Bdellovibrio bacteriovorus is a bacterium that preys upon a wide range of other Gram-negative bacteria, entering their periplasm and consuming them from within. Proteomic and structural analyses of vesicle contents reveal several fibre-like proteins, which we name the mosaic adhesive trimer (MAT) superfamily, and show localization on the predator surface before prey encounter. Structural studies reveal a variety of domain usages (and therefore binding capabilities) at the fibre C-termini, placing these on intertwined trimeric β-prisms. Using independent but complementary approaches, we identified and characterized a MAT superfamily of trimeric fibre proteins with diverse adhesive tips, able to fulfil the long-sought-after role of multiplicity of molecular recognition and handling of diverse epitopes (across a wide prey range), by the bacterial predator B. bacteriovorus.

A region comprising N662 to the C-terminus of Bd2133 was determined to 2.5 Å resolution. The Bd2133 tip is 150 Å long, differentiated into three subdomains —two β-helix regions akin to Bd3182 (G683–E813 and N814–A907) and a β-sandwich domain that substitutes for the S74 chaperone (W913–K1031). The latter two domains are linked by a stalk-like linear peptide (A906AGAAT). Despite a general agreement in the β-helix region, Bd2133 does not possess a Bd3182/S74-like cleft. Equivalents to the Bd3182 capping loops are present, demonstrative of common principles in the S74 and NS74 subgroupings. The β-sandwich tip domain of Bd2133 adopts a twisted fold, trimerizing about strand G989–W999 (burying 5,640 Å2 per monomer). During Bd2133 refinement, we noticed additional density at the sandwich tip, where the trimer interface creates a pocket using Y985, N956 and N1020. Guided by crystal symmetry, we have modelled this as an N-terminal hexapeptide derived from a nearby copy. Negative-stain electron microscopy of full-length Bd2133 (residues 21–1,031) confirmed fibre formation, with dimensions commensurate with an AlphaFold18 model and our partial structural determination, showing fibre conformational flexibility.

>[2x]GSSGALGLSTSGSERMRIDTSGNLGLGTAAPTSALHVERTQDADTTVQVRNTHDTGTAAGARFIASNEKSGIWFGISGTSNTNTGLGSPGDAYIYNAAGTATGKNLNVINNQTGNIHFFAGSTATGTPRMTITNTGLVGINTAAPLQKLHVENGNMVITGTAPAYQLKENDTTDQNWQMGINNGNLRFATQNDALNSSSDKVVISQAGNVGIGATAPTAKLEVAGTIHSTSGGIKFPDGSVQTTAASGAATWTSLGLTSLGAVSMTTTTEQSFTLPVAAQTASQILVYLRCHSGNASTTGADDIRIYTKEGAATYDHYLLMFPYAGQGAVGYNSDSFWLPKTSDNKIYLAHSMAPGSANSGCNFYITGYK> PVMKTFKEFLLSLDDSVDETEAVKRYNDYKLDFRRQQMQDFFLAHKDEEWFRSKYHPDEVGKRRQEARGALQNRLRVFLSLMETGWFDNLLLDI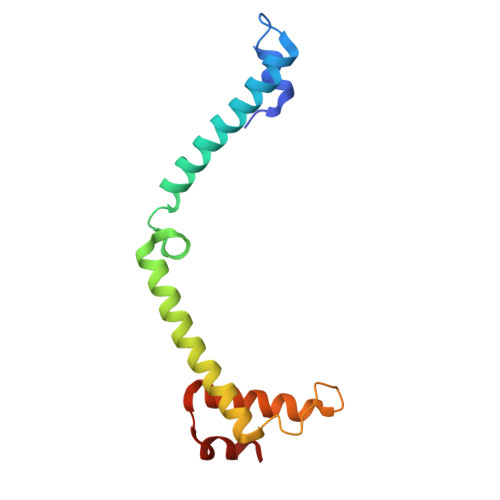DKADAIVKMLDAAVIKMEGGTENDLRILEQ>[6x]MNNKGSGLTPAQALDKLDALYEQSVVALRNAIGNYITSGELPDENARKQGLFVYPSLTVTWDGSTTNPPKTR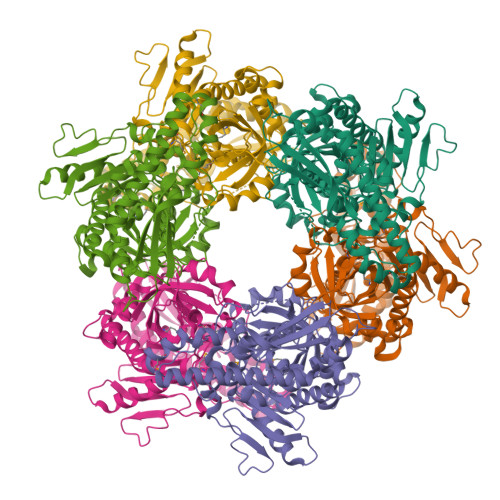AFGRFTHAGSYTTTITRPTLFRSYLNEQLTLLYQDYGAHISVQPSQHEIPYPYVIDGSELTLDRSMSAGLTRYFPTTELAQIGDETADGIYHPTEFSPLSHFDARRVDFSLARLRHYTGTPVEHFQPFVLFTNYTRYVDEFVRWGCSQILDPDSPYIALSCAGGNWITAETEAPEEAISDLAWKKHQMPAWHLITADGQGITLVNIGVGPSNAKTICDHLAVLRPDVWLMIGHCGGLRESQAIGDYVLAHAYLRDDHVLDAVLPPDIPIPSIAEVQRALYDATKLVSGRPGEEVKQRLRTGTVVTTDDRNWELRYSASALRFNLSRAVAIDMESATIAAQGYRFRVPYGTLLCVSDKPLHGEIKLPGQANRFYEGAISEHLQIGIRAIDLLRAEGDRLHSRKLRTFNEPPFR CAP is a 210-amino-acid transcription factor that binds cAMP generated by adenylyl cyclase in response to the phosphorylated form of Enzyme IIAGlc (phosphorylated in response to the phosphoenolpyruvate-carbohydrate phosphotransferase system). cAMP-bound CAP regulates the transcription of over 100 genes crucial for carbon utilization through its binding to a specific promoter region and recruitment of RNA polymerase. Previous studies of the ligand binding domain of CAP demonstrated negative cooperativity between cAMP binding sites in the absence of structural change within this domain. We produce coarse-grained models that describe global low-frequency protein backbone motions of CAP and show a strong correlation between negative cooperativity for cAMP and modulation of the delocalised normal modes on ligand binding without a requirement for a spatially distinct physical pathway or conformational change. We demonstrate experimentally that altered connectivity between backbone elements in CAP can give predictable alterations to cooperativity for cAMP binding through altered mode amplitudes.

Altering local interactions associated with V140 was predicted by the ENM to have minimal effects on cooperativity despite significant local hydrophobic interactions; we therefore examined the effect of decreased and increased local hydrophobic interactions in V140A and V140L variants as a control experiment. Interestingly, although V140A protein showed no global change in structure, there is, in this mutation, a significant local conformational change evident in the crystal structure where the mutated V140A residue formed a new hydrophobic contact with the rotated side chain of C179 that is not present in the wild-type or V140L proteins. ITC experiments demonstrated that this CAP variant with the identified side chain rearrangement was positively cooperative, thus supporting the qualitative prediction of the model.

>[6x]MRGSHHHHHHGSMVLGKPQTDPTLEWFLSHCHIHKYPSKSTLIHQGEKAETLYYIVKGSVAVLIKDEEGKEMILSYLNQGDFIGELGLFEEGQERSAWVRAKTACEVAEISYKKFRQLIQVNPDILMRLSAQMARRLQVTSEKVGNLAFLDATGRIAQTLLNLAKQPDAMTHPDGMQIKITRQEIGQIVGCSRETVGRILKMLEDQNLISAHGKTIVVYGTR>MAYRKRGARRETNLKQDERMQEKEDSKNINNDSPKSQLSEKVLSKKEEIITDNQEEVKISDEVKKSNKEESKQLLEVLKTKEEHQKEVQYEILQKTIPTFEPKESILKKLEDIKPEQAKKQTKLFRIFEPKQLPIYRANGERELRNRWYWKLKRDTLPDGDYDVREYFLNLYDQVLMEMPDYLLLKDMAVENKNSRDAGKVVDSETAAICDAIFQDEETEGAVRRFIAEMRQRVQADRNVVNYPSILHPIDHAFNEYFLQHQLVEPLNNDIIFNYIPERIRNDVNYILNMDRNLPSTARYIRPNLLQDRLNLHDNFESLWDTITTSNYILARSVVPDLKELVSTEAQIQKMSQDLQLEALTIQSETQFLTGINSQAANDCFKTLIAAMLSQRTMSLDFVTTNYMSLISGMWLLTVIPNDMFIRESLVACQLAIINTIVYPAFGMQRMHYRNGDPQTPFQIAEQQIQNFQVANWLHFVNYNQFRQVVIDGVLNQVLNDNIRNGHVVNQLMEALMQLSRQQFPTMPVDYKRSIQRGILLLSNRLGQLVDLTRLLSYNYETLMACITMNMQHVQTLTTEKLQLTSVTSLCMLIGNATVIPSPQTLFHYYNVNVNFHSNYNERINDAVAIITAANRLNLYQKKMKSIVEDFLKRLQIFDVARVPDDQMYRLRDRLRLLPVEIRRLDIFNLIAMNMEQIERASDKIAQGVIIAYRDMQLERDEMYGYVNIARNLDGFQQINLEELMRSGDYAQITNMLLNNQPVALVGALPFITDSSVISLIAKLDATVFAQIVKLRKVDTLKPILYKINSDSNDFYLVANYDWIPTSTTKVYKQVPQQFDFRASMHMLTSNLTFTVYSDLLAFVSADTVEPINAVAFDNMRIMNEL[2x];>[13x]MDVLYSLSKTLKDARDKIVEGTLYSNVSDLIQQFNQMIITMNGNEFQTGGIGNLPIRNWNFNFGLLGTTLLNLDANYVETARNTIDYFVDFVDNVCMDEMVRESQRNGIAPQSDSLRKLSAIKFKRINFDNSSEYIENWNLQNRRQRTGFTFHKPNIFPYSASFTLNRSQPAHDNLMGTMWLNAGSEIQVAGFDYSCAINAPANIQQFEHIVPLRRVLTTATITLLPDAERFSFPRVINSADGATTWFFNPVILRPNNVEVEFLLNGQIINTYQARFGTIVARNFDTIRLSFQLMRPPNMTPAVAVLFPNAQPFEHHATVGLTLRIESAVCESVLADASETLLANVTSVRQEYAIPVGPVFPPGMNWTDLITNYSPSREDNLQRVFTVASIRSMLIK;>[13x]MYGIEYTTVLTFLISIILLNYILKSLTRIMDFIIYRFLFIIVILSPFLRAQNYGINLPITGSMDTAYANSTQEETFLTSTLCLYYPTEAATEINDNSWKDTLSQLFLTKGWPTGSVYFKEYTNIASFSVDPQLYCDYNVVLMKYDATLQLDMSELADLILNEWLCNPMDITLYYYQQTDEANKWISMGSSCTIKVCPLNTQTLGIGCLTTDATTFEEVATAEKLVITDVVDGVNHKLDVTTATCTIRNCKKLGPRENVAVIQVGGSDILDITADPTTAPQTERMMRINWKKWWQVFYTVVDYVDQIIQVMSKRSRSLNSAAFYYRV

The infectivity of rotavirus (RV), the leading cause of childhood diarrhea, hinges on the activation of viral particles through the proteolysis of the spike protein by trypsin-like proteases in the host intestinal lumen. The RV virion is an icosahedral triple layered particle in which the segmented viral genome and the polymerase complexes are packaged in a capsid made of the VP2 protein. The external layer is formed by trimers of the VP7 glycoprotein in phase with the underlaying VP6 shell and 60 trimeric VP4 spikes, which project from the VP7 layer, that clamps them and partially covers their base. This outer layer is responsible for the first steps of RV infection: attachment to cell surface receptors, lipid bilayer penetration, and release of the double-layered particle (DLP) into the cytosol, where transcription of the viral genome is initiated.

To obtain high-resolution maps of activated and inactivated particles, TLP from cells infected with rotavirus in the presence of trypsin (TR-TLP), or in its absence in medium supplemented with the protease inhibitor leupeptin (NTR-TLP), were purified by density gradient ultracentrifugation and characterized by SDS-PAGE. In contrast, for the TR-TLP, the proteolytic products VP8* (28 kDa) and VP5* (55 kDa) were detected as two distinct bands. Three-dimensional reconstructions (3DR) of NTR- and TR-TLP were computed using SPA with imposition of icosahedral symmetry, achieving resolutions of 3.40 Å and 3.48 Å for NTR- and TR-TLP, respectively. While the density of the VP2, VP6 and VP7 shells exhibited a homogeneous high local resolution, the spike showed a radial decrease in resolution as it extended away from the outer shell surface, with particularly low resolution in the body and head regions. The resulting maps provided sufficient quality to support full atomic modelling in the foot and stalk domains, while in the body and head regions, a combination of backbone tracing and rigid-body fitting was applied (representative examples of model-to-map fitting for each region are shown in S8 Fig). These enhanced densities, together with the icosahedral 3DR of the complete NTR and TR TLPs, were used to build and refine the full asymmetric subunits, including all VP2, VP4, VP6, and VP7 chains.>HHHHHHMRTANLYLAGIGSHLPPLFPAERAVAEGLYDEEARQSSGMRSAAVSASTPAPQMAIDAARAALESSGHDADDIGILLHSYTHHQGPDGWSAVHYILNNTVDRPVPAVEIKQGCLGMLASLDVAAARLIANPTHDAALITTGDNYSTPGVERWRASGLFVLADAGSAVVLSRRGGFAELLALDSLSDSSMEILHRAGEELFPPGVTRGRGLNFAERAEKVREQWAAGQAPPIKNFGDRVAEVTERVLKQADVSWDQIAKVCHV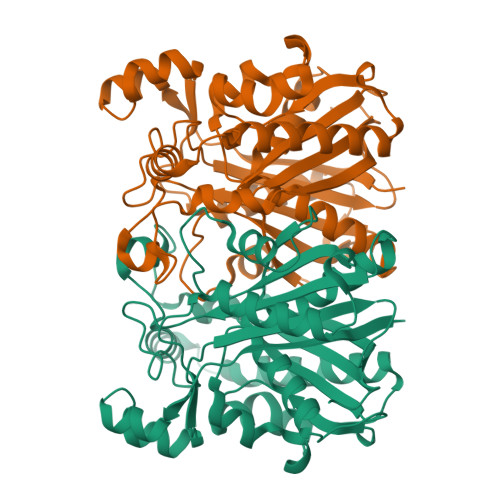GFGRPALEAMFLLPLDVPEEKTVWEYANTIGHTGAADLFLGLEHVWRTGQVGPGDHVLLIGASTGMEAGAAVVRIAEAAPGSQGGGDA[2x]>[2x]MAIGEFMVSLPRMVYPQPKVLTPCRKDVLVVTPWLAPIVWEGTFNIDILNEQFRLQNTTIGLTVFAIKKYVAFLKLFLETAEKHFMVGHRVHYYVFTDQPAAVPRVTLGTGRQLSVLEVRAYKRWQDVSMRRMEMISDFCERRFLSEVDYLVCVDVDMEFRDHVGVEILTPLFGTLHPGFYGSSREAFTYERRPQSQAYIPKDEGDFYYGGAFFGGSVQEVQRLTRACHQAMMVDQANGIEAVWHDESHLNKYLLRHKPTKVLSPEYLWDQQLLGWPAVLRKLRFTAVPKNHQAVRNP

One important example is the biosynthesis of human ABO blood group antigens, which is the most important blood group system in transfusion and transplantation. GTA catalyzes the transfer of GalNAc from UDP-GalNAc to the H antigen acceptor (HAA) (α-l-Fuc-(1→2)-β-d-Gal-O-R, where R is glycolipid or glycoprotein) to form the A antigen, whereas GTB catalyzes the transfer of Gal from UDP-Gal to the HAA to form the B antigen. Among these is the enzyme AAGlyB, a dual-specificity GT, which can bind and utilize either UDP-Gal or UDP-GalNAc with equal efficiency. Each letter corresponds to one critical residue in increasing order such that the AAGlyB chimer would correspond to GTA-L266G/G268A.

In the AAGlyB-2 and AAGlyB-2-HAA complexes where the 5-substituent of the donor analogue is a phenyl group, the electron density is well defined throughout most of the only chain in the AAGlyB-2 structure and chain A and B in the AAGlyB-2-HAA structure. In the AAGlyB-2-HAA structure, upon binding of the acceptor, the internal loop also goes from a disordered state in the “donor-only” complex to an ordered closed conformation with Trp-181 stacking to the phenyl substituent of 2. However, compared with the AAGlyB-1-HAA complex the internal loop of the B chain of AAGlyB-2-HAA is slightly less ordered, and residues 196–198 are missing entirely. Furthermore, in the AAGlyB-2-HAA structure the C terminus of both chain A and B in the asymmetric unit does not fold over the binding site in the same way as seen in chain A of the AAGlyB-1-HAA complex and is only visible until residue 346. Also, the lack of electron density of the C terminus cannot be explained by poor data resolution because AAGlyB-2-HAA diffracted to 1.7 Å whereas AAGlyB-1-HAA diffracted to only 1.9 Å. Therefore, the reason for the destabilization of the C terminus and of the internal loop in chain B in the presence of 2 is likely the lack of hydrogen bonding to Val-351, of the type observed for the formylthienyl substituent in 1. Finally, as for the AAGlyB-1 structure, the AAGlyB-2 shows well defined density for the galactose in the tucked under conformation, whereas in the AAGlyB-2-HAA structure the galactose is not visible except for a few blobs extending out from the nucleotide β-phosphate. This suggests that, although our enzyme kinetics results show a lower turnover number for compound 2 compared with compound 1, and although the C terminus seems to be incapable of folding over the active site, the enzyme is still slowly hydrolyzing the donor derivative when soaked into the crystal. Our results suggest that this pseudo-closed conformation allows the transfer of the sugar, albeit at a slower rate than the native, closed conformation, and could therefore be the reason for the small, residual turnover observed for AAGlyB toward 1.> GDELYRQSLEIISRYLREQATGAKDTKPMGRAGATSRKALETLRRVGDGVQRNHETAFQGMLRKLDIANEDDVKSLSRVMIHVFSDGVTNW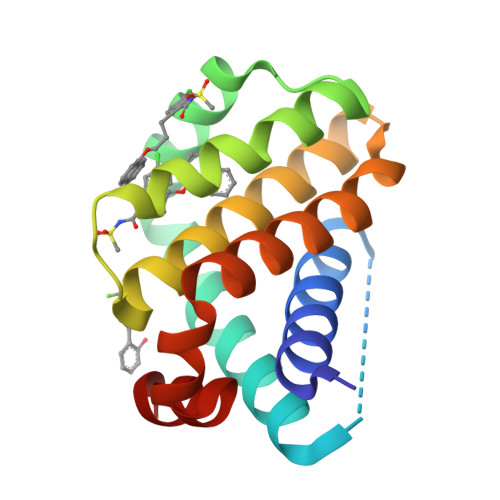GRIVTLISFGAFVAKHLKTINQESCIAPLAESITDVLVRTKRDWLVAQRGWDGFVEFFH> NNNGACUUAAGUCGG;> NNNG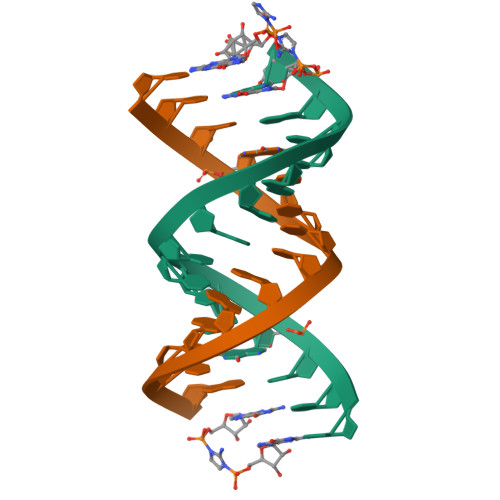ACUUAAGUCG1-[7-[1,5-dimethyl-3-(phenoxymethyl)pyrazol-4-yl]-3-(3-naphthalen-1-yloxypropyl)-1~{H}-indol-2-yl]-2,2-bis(oxidanyl)ethanone | C35 H33 N3 O5 | 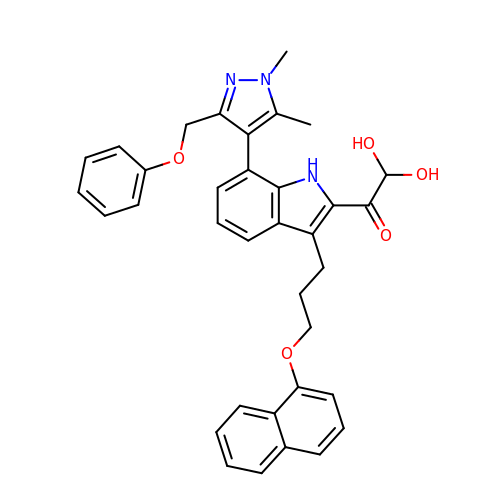WZCPCAOYSVDSOO-UHFFFAOYSA-N> GPLGSMEGLFSQKSFLVLGFSVENKCNIVDIIREHAGKIVSLPSRIVADYAVVPLLGCEVDVTVGEVVTNTWLVTCIDNQTLVDPKSNPLFTPVSVMSGVTPLEDCVISFSQCVGAERDSLVFLANHLGASVQEFFVRKANAKKGMLASTHLIVKEPTGSKYEAAKKWSLPAVN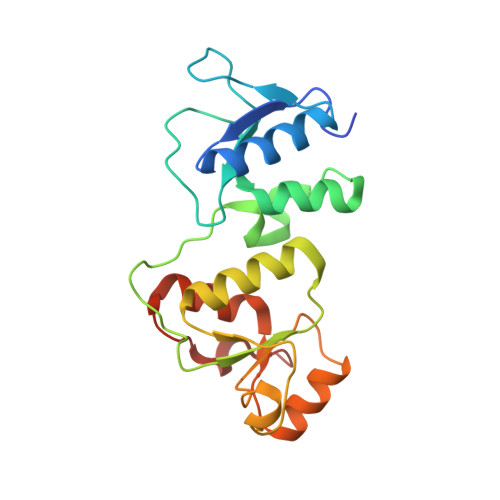ISWLLETARIGKRADENHFLVDNAPK> LYHTVPPAVVGVGGGGVNAGPVASGAIVGTNGYVITTLHSVSKLPEISVQVATTGGIRRFPAQVVKTIPGHDLALLKMQTTEKFLHFRMADVQTVVPGQQVFAFGRNMAGAPLVRQGLVQSADAPLAVGATQITHLLRSDAVYSWEQTGGPLVNAQGDLVGINIAATGPTGKVEGFTVPAQVIVSHLQDVV

Here, we characterize a protein called MamO that helps to initiate the formation of a magnetic mineral called magnetite in cells of the magnetotactic bacterium Magentospirillum magneticum AMB-1. Although predicted to be a trypsin-like protease, we show that MamO has lost its ancestral catalytic activity and instead gained a new function as a metal-binding scaffold. Two genes in the MAI, mamE and mamO, are homologous to the HtrA proteases, a ubiquitous family of trypsin-like enzymes that functions using His-Asp-Ser catalytic triads. It appears to have lost the ability to perform serine protease activity and instead performs two noncatalytic functions: direct metal binding to promote magnetite nucleation and activation of MamE’s proteolytic activity.

Although the MamO crystals grow in acidic conditions that disfavor metal binding, they could be soaked at pH 8.0 without affecting diffraction. We solved another structure of the protease domain using crystals soaked in NiCl2 at pH 8.0 and identified a metal binding site. Overall, the conformation of the protease domain is highly similar to the original structure (root-mean-square deviation of 0.17 Å over 184 residues), and it contains the unidentified peptide. Additionally, a single Ni2+ ion binds between loop LC and helix 2, with H148 and H263 directly coordinating the metal. We confirmed the placement of the ligand at this site using single wavelength anomalous dispersion (SAD) data collected at the Ni absorption edge. MamO’s di-histidine motif is highly reminiscent of the Zn2+ binding site in another trypsin-like protease, kallikrein-3, in which Zn2+attenuates protease activity by altering the position of catalytic triad residues H57 and D102. Taken together, our biochemical and structural investigations show that MamO binds to transition metal ions using H148 and H263, but that metal binding is not restricted to this motif. We conclude that H148 and H263 contribute to a metal binding function that is required for magnetite nucleation in vivo. Interestingly, H116 and D149 participate in a hydrogen bond on the opposite face of loop LC from the H148/H263 metal binding motif, suggesting that the conditional phenotypes could be due to temperature-dependent flexibility near the metal binding site. It appears that binding is insufficient and that the precise coordination geometry must be maintained, leading us to speculate that MamO directly promotes nucleation by guiding individual iron atoms into the magnetite lattice.> AEGKLNDELAKNKGKIPGLKIDQKIRGQMPEQGWTEDDIKNTVSNGATGTSFDKRSPKKTPPDYLGRNDPATVYGSPGKYVVVNDRTGEVTQISD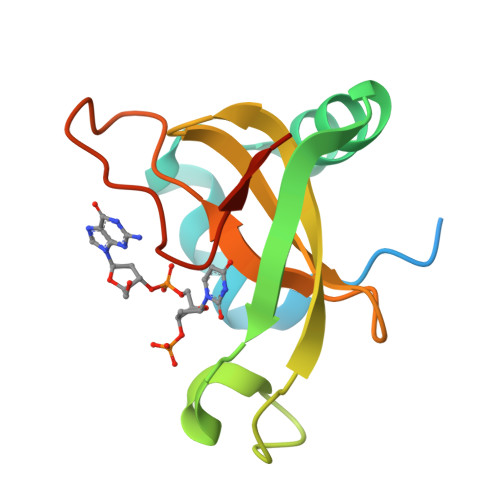KTDPGWVDDSRIQWGNKNDQ4-[(2-azanyl-4-oxidanylidene-7,8-dihydro-3~{H}-pteridin-6-yl)methylamino]-~{N}-(5,6-dimethoxypyrimidin-4-yl)benzenesulfonamide 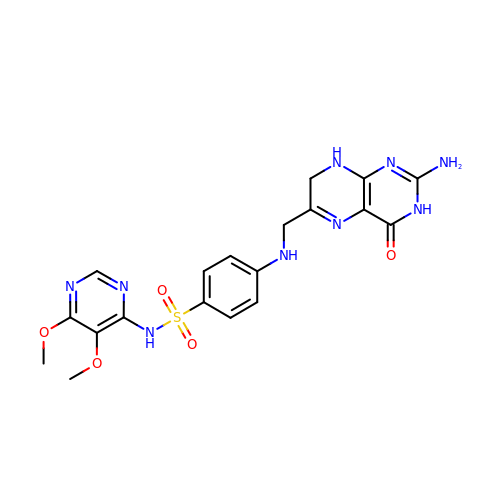| C19 H21 N9 O5 S | YQBRQWRFWGQPMG-UHFFFAOYSA-N> GPMGALTKAEIAERLYEELGLNKREAKELVELFFEEIRQALEHNEQVKLSGFGNFDLRDKRQRP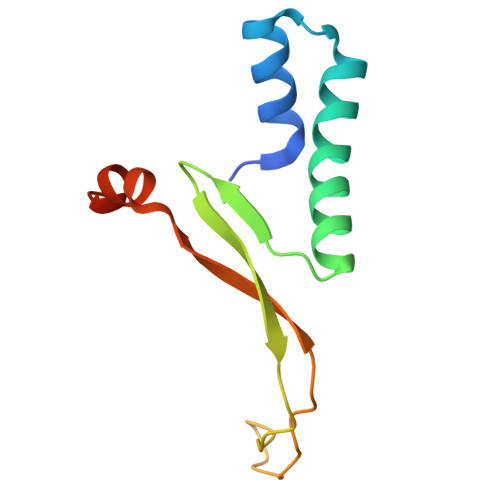GRNPKTGEEIPITARRVVTFRPGQKLKARVEAYAGTKS ethyl (4R)-4-[[(2S,3R)-1-[(2S)-3-methyl-2-[(5-methyl-1,2-oxazol-3-yl)carbonylamino]butanoyl]-3-phenyl-pyrrolidin-2-yl]carbonylamino]-5-[(3S)-2-oxidanylidenepyrrolidin-3-yl]pentanoate 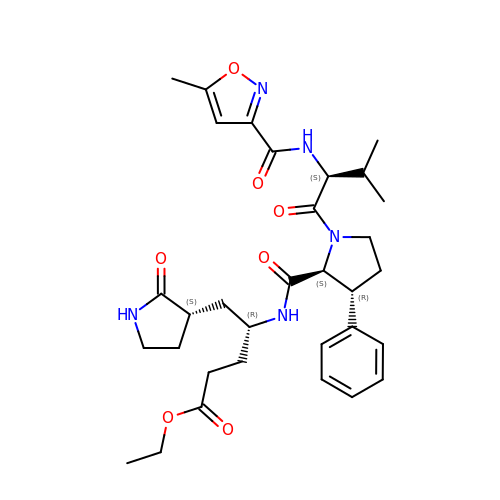| C32 H43 N5 O7 | CVLPPZUDRJEOCI-RTOJZCGHSA-N methyl 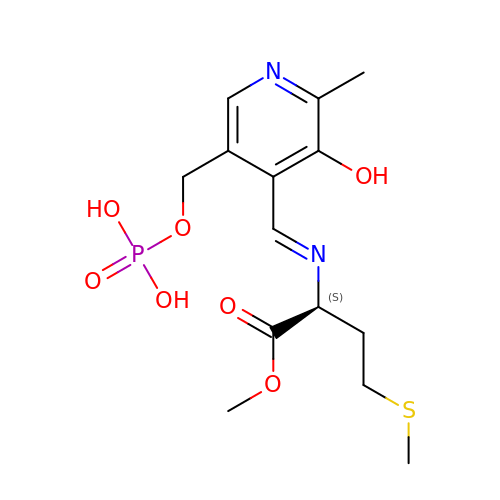(2S)-2-[(E)-[2-methyl-3-oxidanyl-5-(phosphonooxymethyl)pyridin-4-yl]methylideneamino]-4-methylsulfanyl-butanoate | C14 H21 N2 O7 P S | VXNUIRDVLGPXAG-QFULYMJESA-N The bacterial flagellar motor is a huge bidirectional rotary nanomachine that drives rotation of the flagellum for bacterial motility. The cytoplasmic C ring of the flagellar motor functions as the switch complex for the rotational direction switching from counterclockwise to clockwise. The basal body is made up of the LP ring, MS ring, C ring, rod and export apparatus. Here, we present two high-resolution cryo-electron microscopy structures of the C ring-containing flagellar basal body–hook complex from Salmonella Typhimurium, which are in the default counterclockwise state and in a constitutively active CheY mutant-induced clockwise state, respectively.

To obtain the C ring-containing basal body–hook complex in the CW state, we constructed the constitutively active double mutant D13K/Y106W of CheY (hereafter referred to as CheY**), which can mimic CheY-P to tightly bind to the C ring and lock the rotational direction of the motor in the CW state. The density maps of the LP ring, MS ring, rod, hook, and export apparatus in the CW state were locally reconstructed to the higher resolutions ranging from 2.8 Å to 3.8 Å. Although the structures of the LP ring, MS ring, rod, hook, and export apparatus in the CW state are highly similar to those of these components in the CCW state, the protomers of the C ring in the CW state notably undergo inclination and compaction, suggesting that the binding of CheY** induces significant conformational changes of the C ring for rotational switching. The LP ring acts as a bushing to stabilize the rotation of the rod, which serves as the drive shaft.

>[26x]MQKYALHAYPVMALMVATLTGCAWIPAKPLVQGATTAQPIPGPVPVANGSIFQSAQPINYGYQPLFEDRRPRNIGDTLTIVLQENVSASKSSSANASRDGKTSFGFDTVPRYLQGLFGNSRADMEASGGNSFNGKGGANASNTFSGTLTVTVDQVLANGNLHVVGEKQIAINQGTEFIRFSGVVNPRTISGSNSVPSTQVADARIEYVGNGYINEAQNMGWLQRFFLNLSPM;>[26x]MFKALAGIVLALVATLAHAERIRDLTSVQGVRENSLIGYGLVVGLDGTGDQTTQTPFTTQTLNNMLSQLGITVPTGTNMQLKNVAAVMVTASYPPFARQGQTIDVVVSSMGNAKSLRGGTLLMTPLKGVDSQVYALAQGNILVGGAGASAGGSSVQVNQLNGGRITNGAIIERELPTQFGAGNTINLQLNDEDFTMAQQITDAINRARGYGSATALDARTVQVRVPSGNSSQVRFLADIQNMEVNVTPQDAKVVINSRTGSVVMNREVTLDSCAVAQGNLSVTVNRQLNVNQPNTPFGGGQTVVTPQTQIDLRQSGGSLQSVRSSANLNSVVRALNALGATPMDLMSILQSMQSAGCLRAKLEII9-(4-HYDROXYBUTYL)-N2-PHENYLGUANINE | C15 H17 N5 O2 | 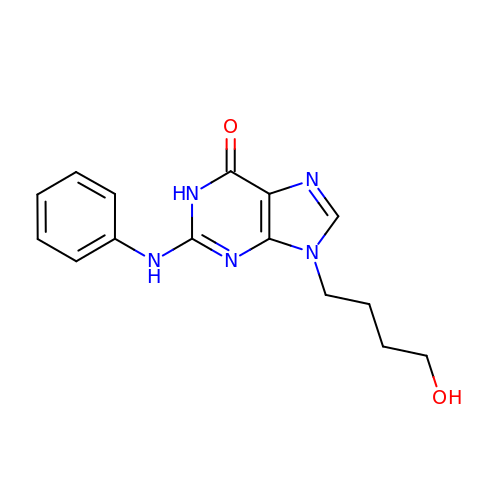JHBXNPBKSPYOFT-UHFFFAOYSA-N Icilin | C16 H13 N3 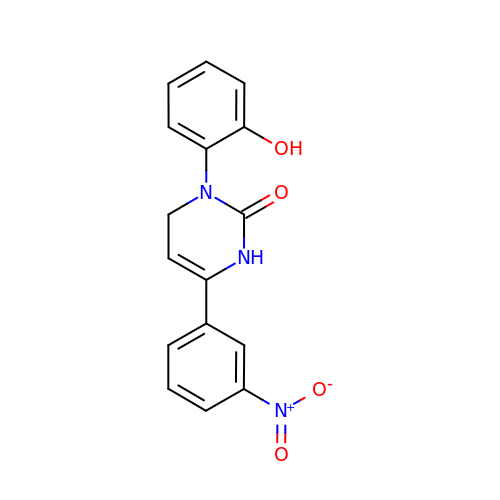O4 | RCEFMOGVOYEGJN-UHFFFAOYSA-N>[1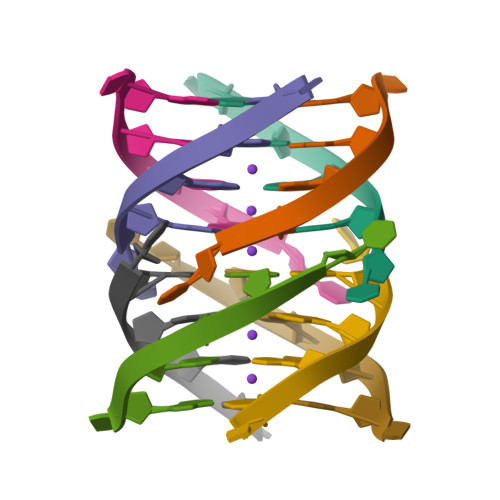6x]TGGGGT>MPELPEVEAARRAIEENCLGKKIKRVIIADDNKVIHGISPSDFQTSILGKTIISARRKGKNLWLELDSPPFPSFQFGMAGAIYIKGVAVTKYKRSAVKDSEEWPSKYSKFFVELDDGLELSFTDKRRFAKVRLLANPTSVSPISELGPDALLEPMTVDEFAESLAKKKITIKPLLLDQGYISGIGNWIADEVLYQARIHPLQTASSLSKEQCEALHTSIKEVIEKAVEVDADSSQFPSNWIFHNREKKPGKAFVDGKKIDFITAGGRTTAYVPELQKL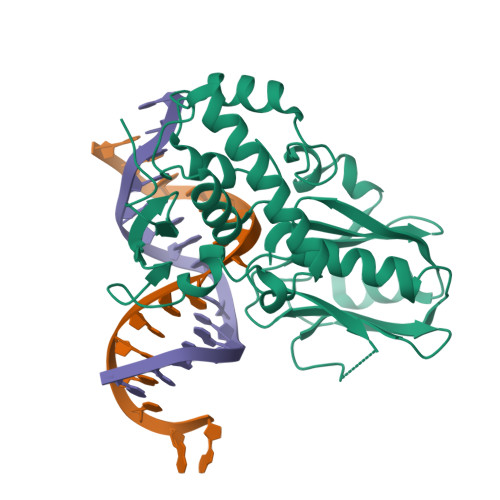YGKDAEKAAKVRPAKRGVKPKEDDGDHHHHHH[2x]methyl 2-(4-chloranylindol-1-yl)-2-oxidanylidene-ethanoate 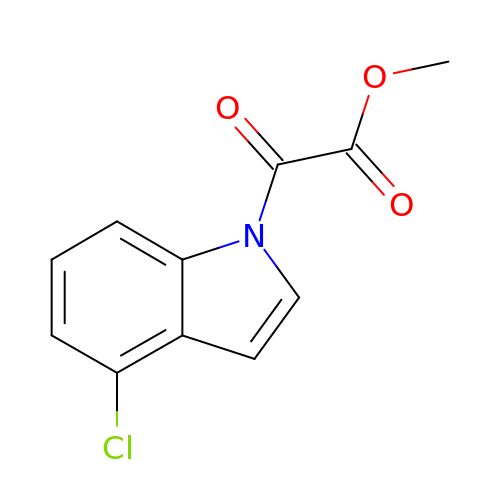| C11 H8 Cl N O3 | QRAIXQAFCRLHNQ-UHFFFAOYSA-N> TTPLVHVASVEKGRSYEDFQKVYNAIALKLREDDEYDNYIGYGPVLVRLAWHTSGTWDKHDNTGGSYGGTYRFKKEFNDPSNAGLQNGFKFLEPIHKEFPWISSGDLFSLGGVTAVQEMQGPKIPWRCGRVDTPEDTTPDNGRLPDADKDADYVRTFFQRL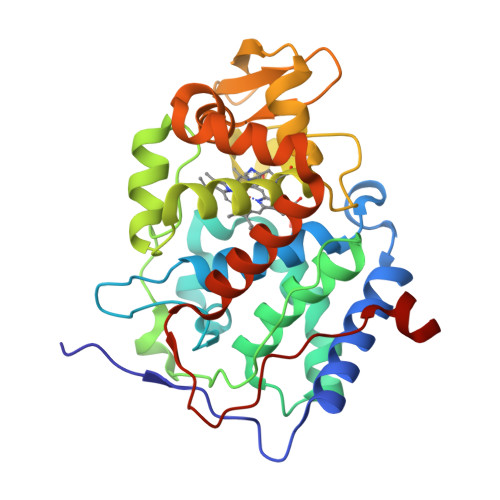NMNDREVVALMGAHALGKTHLKRSGYEGPWGAANNVFTNEFYLNLLNEDWKLEKNDANNEQWDSKSGYMMLPTDYSLIQDPKYLSIVKEYANDQDKFFKDFSKAFEKLLENGITFPKDAPSPFIFKTLEEQGL>[2x]SMIVLF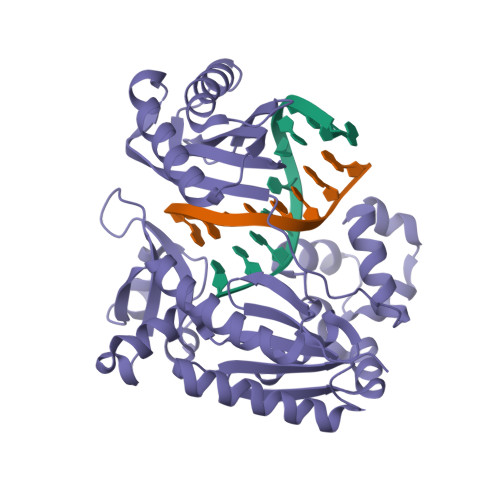VDFDYFYAQVEEVLNPSLKGKPVVVCVFSGRFEDSGAVATANYEARKFGVKAGIPIVEAKKILPNAVYLPMRKEVYQQVSSRIMNLLREYSEKIEIASIDEAYLDISDKVRDYREAYNLGLEIKNKILEKEKITVTVGISKNKVFAKIAADMAKPNGIKVIDDEEVKRLIRELDIADVPGIGNITAEKLKKLGINKLVDTLSIEFDKLKGMIGEAKAKYLISLARDEYNEPIRTRVRKSIGRIVTMKRNSRNLEEIKPYLFRAIEESYYKLDKRIPKAIHVVAVTEDLDIVSRGRTFPHGISKETAYSESVKLLQKILEEDERKIRRIGVRFSKFI> MGSSHHHHHHQQVSLQPPPQQLIVQNKTIDLPAVYQLNGGEEANPHAVKVLKELLSGKQSSKKGMLISIGEKGDKSVRKYSRQIPDHKEGYYLSVNEKEIVLAGNDERGTYYALQTFAQLLKDGKLPEVEIKDYPSVRYRGVVEGFYGTPWSHQARLSQLKFYGKNKMNTYIYGPKDDPYHSAPNWRLPYPDKEAAQLQELVAVANENEVDFVWAIHPGQDIKWNKEDRDLLLAKFEKMYQLGVRSFAVFFDDISGEGTNPQKQAELLNYIDEKFAQVKPDINQLVMCPTEYNKSWSNPNGNYLTTLGDKLNPSIQIMWTGDRVISDITRDGISWINERIKRPAYIWWNFPVSDYVRDHLLLGPVYGNDTTIAKEMSGFVTNPMEHAESSKIAIYSVASYAWNPAKYDTWQTWKDAIRTILPSAAEELECFAMHNSDLGPNGHGYRREESMDIQPAAERFLKAFKEGKNYDKADFETLQYTFERMKESADILLMNTENKPLIVEITPWVHQFKLTAEMGEEVLKMVEGRNESYFLRKYNHVKALQQQMFYIDQTSNQNPYQPGVKTATRVIKPLIDRTFATVVKFFNQKFNAHLDATTDYMPHKMISNVEQIKNLPLQVKANRVLISPANEVVKWAAGNSVEIELDAIYPGENIQINFGKDAPCTWGRLEIS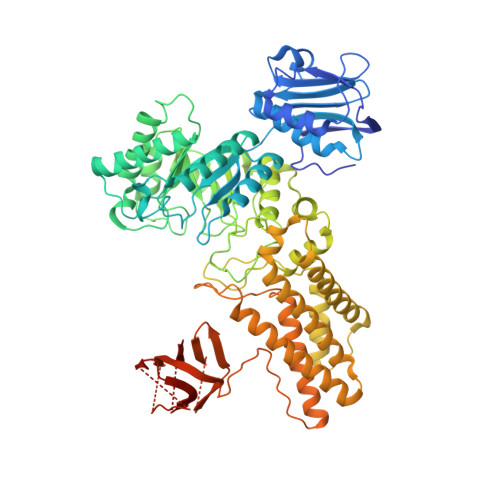TDGKEWKTVDLKQKESRLSAGLQKAPVKFVRFTNVSDEEQQVYLRQFVLTIEKK> AGGCGCAUUUGAACUGUAUUGUACGCCUUGCAUAAAGCAAAAGUACUAAAAAA

SAM-V is one of the class of riboswitches that bind S-adenosylmethione, regulating gene expression by controlling translation. Breaker and co-workers described a new class of SAM riboswitches called SAM-V, that was found by bioinformatic analysis of intergenic regions of marine α-protobacteria and bacteroidetes. The RNA folds as an H-type pseudoknot, with a major-groove triple helix in which resides the SAM ligand binding site. We propose a model in which SAM binding leads to association of the triplex third strand that stabilizes a short helix and occludes the ribosome binding site.

We have solved the crystal structure of the metY SAM-V riboswitch bound to its SAM ligand at 2.5 Å resolution. A 53-nt RNA corresponding to the metY SAM-V riboswitch from Candidatus Pelagibacter ubique was made by chemical synthesis. This included one 5-bromocytosine nucleotide at position 4 that was used to provide phase information by means of its anomalous scattering. The RNA was co-crystallized with SAM, in space group P4122. The chain of the SAM ligand bound to the riboswitch is maximally extended and aligned with the helical axis. The adenine nucleobase of SAM is basepaired with U47 as a trans Hoogsteen basepair, with hydrogen bonds from N6 to U47O2 and from U47N3 to N7. At the other end of the SAM chain the aminoacyl group is hydrogen bonded to the nucleobase of A50, donating a proton from N6 to the carboxyl O and accepting one at N1 from the amine. The carboxyl group makes additional contacts to a hydrated metal ion that is bound site-specifically to the RNA; the metal-O distance is 2.1 Å, so this is most likely a Mg2+ ion. The SAM sulfonium is coplanar with the U20:A48.U9 base triple, lying on the helical axis and thus surrounded by the triple on one side. The positively charged sulfur atom is 3.2 and 3.3 Å from the O4 carbonyl atoms of U20 and U9.[4-({[5-BENZYLOXY-1-(3-CARBAMIMIDOYL-BENZYL)-1H-INDOLE-2-CARBONYL]-AMINO}-METHYL)-PHENYL]-TRIMETHYL-AMMONIUM | 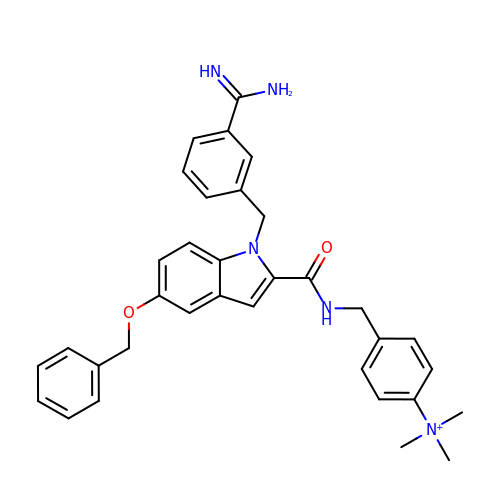C34 H36 N5 O2 | UFKJQTGPBFWMGT-UHFFFAOYSA-O>[2x]MNAVEIQGVSQRYGSMTVLHDLNLNLGEGEVLGLFGHNGAGKTTSMKLILGLLSPSEGQVKVLGRAPNDPQVRRQLGYLPENVTFYPQLSGRETLRHFARLKGAALTQVDELLEQVGLAHAADRRVKTYSKGMRQRLGLAQALLGEPRLLLLDEPTVGLDPI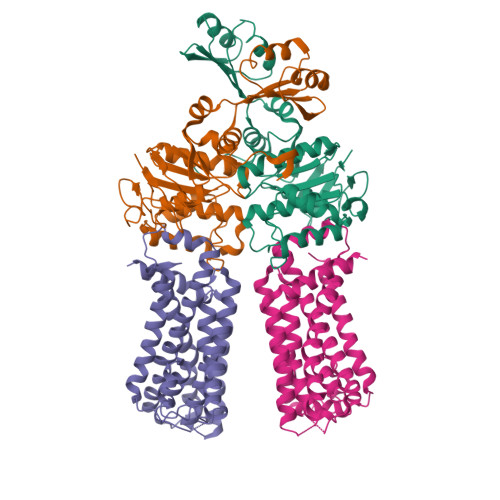ATQDLYLLIDRLRQRGTSIILCSHVLPGVEAHINRAAILAKGCLQAVGSLSQLRAEAGLPVRIRASGISERDSWLQRWTDAGHSARGLSESSIEVVAVNGHKLVLLRQLLGEGEPEDIEIHQPSLEDLYRYYMERAGDVRAQEGRL;>MNQVWNIARKELSDGLRNRWLLAISLLFAVLAVGIAWLGAAASGQLGFTSIPATIASLASLATFLMPLIALLLAYDAIVGEDEGGTLMLLLTYPLGRGQILLGKFVGHGLILALAVLIGFGCAALAIALLVEGVELGMLFWAFGRFMISSTLLGWVFLAFAYVLSGKVNEKSSAAGLALGVWFLFVLVFDLVLLALLVLSEGKFNPELLPWLLLLNPTDIYRLINLSGFEGSGSAMGVLSLGADLPVPAAVLWLCLLAWIGVSLLLAYAIFRRRLT[2x]>ETGKETAFVEVVLFESSPSGDYTTHTTGLTGRFSRAGAMLSAEGEIVQMHPLGLCNNNDEEDLYEYGWVGVVKLEQPELDPKPCLTVLGKAKRAVQRGATAVIFDVSENPEAIDQLNQGSEDPLKRPVVYVKGADAIKLMNIVNKQKVARARIQHLGTKHHHHHH[2x]

Rspo (R-spondin, also roof plate-specific spondin) proteins are evolutionarily conserved from fish to humans and have well-documented roles in a broad range of developmental and physiological processes resulting from enhancement of canonical and non-canonical Wnt signalling. ZNRF3/RNF43 specifically targets these Wnt receptors for ubiquitination and turnover, hence reducing Wnt signalling responses. Direct extracellular interaction with Rspo proteins inhibits ZNRF3/RNF43 activity. Here we report a molecular level analysis of the ZNRF3/RNF43 ectodomain structure and its interactions with Rspo proteins.

The ZNRF3ecto crystal structures revealed a distinctive variant of the protease-associated domain topology. Two β-sheets (comprising β2, β1, β7, β3 and β4, β5, β6 strands, respectively) splay apart, accommodating an α-helix (αC) at the open edge; two additional α-helices (αA and αB) pack against the β4, β5 and β6 face of this distorted β-sandwich. A disulphide bridge, conserved across species, links two structurally elaborate loops, β3–β4 and β4–αA. The crystal structures for apo xZNRF3ecto, zZNRF3ecto and mZNRF3ecto showed no major differences in the main chain conformation. Comparisons of ZNRF3ecto structures for proteins crystallized in several different crystal lattices, or for crystals containing multiple copies in the asymmetric unit, consistently highlighted an acidic region (N105-E114; residue numbering is for mouse sequences unless otherwise stated) within the β3–β4 loop, the short αC–β7 loop and the extended β1–β2 hairpin as flexible elements of the fold. Our crystallographic data provided independent structures for multiple copies of the ZNRF3 ectodomain in eight different crystal forms. All but two of these crystal structures reveal an extensive interface (average interface area 992±109 Å2) formed between two ZNRF3ecto polypeptide chains. This dimer is conserved, and pairwise structural superpositions yielded r.m.s.d. values of <1.3 Å (for 275 equivalent Cα pairs). The interaction is twofold symmetric; strands β3 and β7 of the ‘subunits’ abut face-to-face at the core of the dimer. Intriguingly, these structural features interact in a parallel (cis) fashion consistent with ZNRF3 associating as a dimer on the cell surface.~{N}-[2-(7-methoxynaphthalen-1-yl)ethyl]ethanamide | 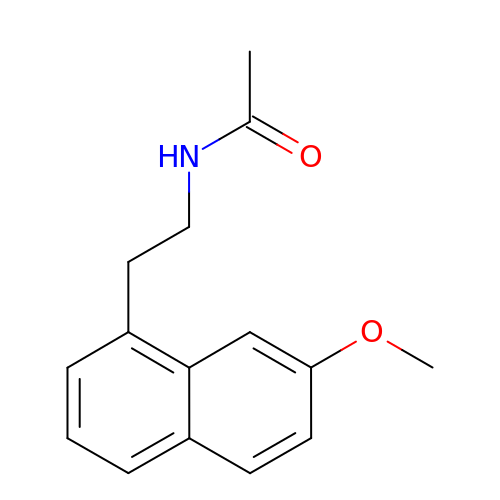C15 H17 N O2 | YJYPHIXNFHFHND-UHFFFAOYSA-N The first step of nitrogen assimilation in higher plants, the energy-driven incorporation of ammonia into glutamate, is catalyzed by glutamine synthetase. Glutamine synthetase (GS; EC 6.3.1.2) is a vital enzyme in the nitrogen metabolism of all living systems. Consistent with the diversity of metabolic roles, GS exists in plants as a number of isoenzymes, located both in the cytosol (GSII-1) and in the plastids (GSII-2), that are encoded by a small gene family. MtGSII-1a is expressed in the vascular bundles of all plant organs and is highly up­regulated in the nodules, accounting for the production of over 90% of the total nodule GS activity.

The three-dimensional structure of M. truncatula GSII-1a was determined at 2.35 Å resolution by X-ray crystallography using synchrotron radiation. The crystallographic model revealed a decameric arrangement of the enzyme with D5 symmetry, with two stacked (face-to-face) pentameric rings. The ten MtGSII-1a monomers adopt very similar conformations, as highlighted by the r.m.s.d. of 0.35–0.65 Å for 291–311 aligned Cα atoms. The extensive contacts established between the subunits that compose each ring result in a buried inter-monomer surface of approximately 3500 Å2. The overall buried inter-ring surface amounts to ∼2500 Å2, i.e. approximately 500 Å2 per individual monomer–monomer interaction, highlighting the weakness of the inter-ring contacts. Considering the contacting monomers A and F from opposed rings, hydrophobic interactions exist between the side chain of Trp141A and both Ile147F and Gly148F, as well as between Gly148A and the side chain of Trp141F. In this particular case, the structure of the apo form of the enzyme was determined and therefore there are no ligands present in any of the ten active centres. In all of the MtGSII-1a monomers a segment comprising the Thr293–Ala299 region, homologous to the Glu-binding loop of bacterial glutamine synthetases, is disordered, leaving open the entrance to the glutamate-binding site at the narrower end of the active-site cavity. Despite the remarkable structural similarity between MtGSII-1a (r.m.s.d. of 0.98–1.03 Å for 320–322 aligned Cα atoms) and its closest structurally characterized homologue, ZmGSII-1a, there are some critical differences between the two enzymes. There is also a concerted movement of several segments of MtGSII-1a, notably the ∼180° rotation of Ala246, with its side chain now protruding into the glutamate-binding pocket, and the ∼90° rotation of the upstream Trp243 side chain that packs against Pro248 and leads to a rearrangement of the Lys237–Asp242 segment.

>[10x]MGSSHHHHHHSSGLVPRGSHASMSLLSDLINLNLSESSEKIIAEYIWVGGSGMDLRSKARTLPGPVSDPSKLPKWNYDGSSTNQAPGQDSEVILYPQAIFKDPFRQGNNILVICDVYTPAGEPLPTNKRYNAAKIFSHPDVAAEVPWYGIEQEYTLLQKDTNWPLGWPIGGYPGPQGPYYCGIGADKAYGRDIVDAHYKACLYAGINISGINGEVMPGQWEFQVGPSVGISAGDEIWAARYILERITEIAGVVVSFDPKPIPGDWNGAGAHTNYSTKSMRENGGYEIIKKAIEKLGLRHKEHIAAYGEGNERRLTGKHETADINTFSWGVANRGASVRVGRDTEKDGKGYFEDRRPSSNMDPYVVTSMIAETTLLWKP> SAGHKVKLAAITCELPARSYENDDPVFAAVPDLSESWWQFWGVNRRGYFDPRNGENEFSLVVRAAERLLRSSDTAPDSVDMLICSASSPIMTDAGDVLPDLRGRLYPRMANVLSKQLGLSRALPLDSQMEAASFLLNLRLAASMIRQGKAEKVLVVCSEYISNLLDFTSRTSTLFADGCAVALLTRGDDDSCDLLASAEHSDATFYEVATGRWRLPENPTGEAKPRLYFSLFSDGQNKMASFVPTNVPIAMRRALEKAGLGSDDIDYFVFHQPAPFLVKAWAEGIGARPEQYQLTMGDTGVMISVSIPYTLMTGL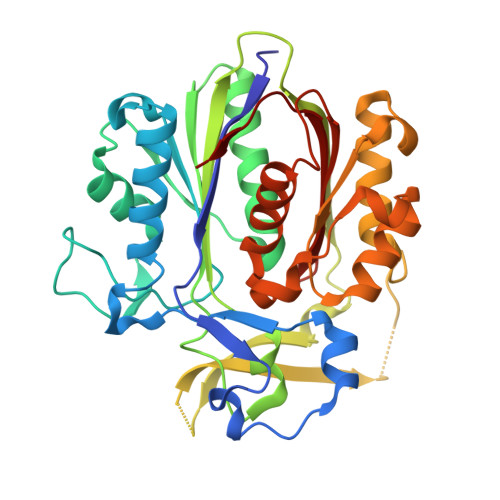REGKIRPGDRIVMAGAATGWGFAAQVWQLGEVLVC>[4x]MAHHHHHHVGTGSNDDDDKSPDPTHNKPLPENVKYGIVLDAGSSHTNLYIYKWPAEKENDTGVVQQLEECQVKGPGISKYAQKTDEIAAYLAECMKMSTERIPASKQHQTPVYLGATAGMRLLRMESKQSA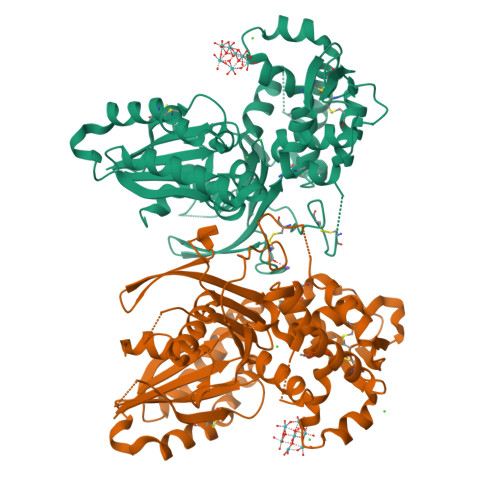DEVLAAVSRSLKSYPFDFQGAKIITGQEEGAYGWITINYLLGRFKTPGGSTFGALDLGGSSTQITFVPLNSTLEAPETSLQFRLYGTDYTVYTHSFLCYGKDQALWQKLAQDIQVSSGGILKDPCFYPGYKKVVNVSELYGTPCTKRFEKKLPFNQFQVQGTGDYEQCHQSILKIFNNSHCPYSQCAFNGVFLPPLQGSFGAFSAFYFVMDFFKKMANDSVSSQEKMTEITKNFCSKPWEEVKASYPTVKEKYLSEYCFSGTYILSLLLQGYNFTGTSWDQIHFMGKIKDSNAGWTLGYMLNLTNMIPAEQPLSPPLPHST>[2x]AFLHVGAQLGTELFIVRQLLQIVKQKTNQNSVDTTLKFTLSALWNLTDESPTTCRHFIENQGLELFMRVLESFPTESS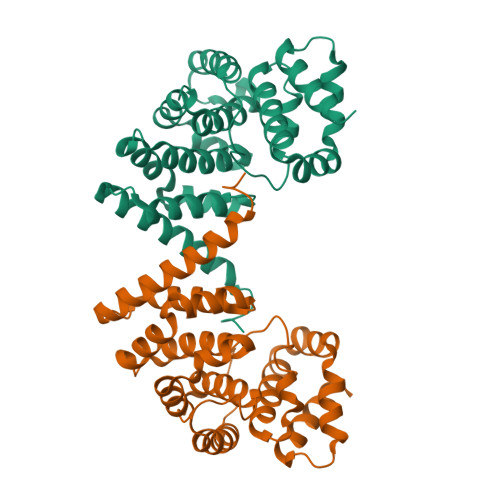IQQKVLGLLNNIAEVQELHSELMWKDFIDHISSLLHSVEVEVSYFAAGIIAHLISRGEQAWTLSRSQRNSLLDDLHSAILKWPTPECEMVAYRSFNPFFPLLGCFTTPGVQLWAVWAMQHVCSKNPSRYCSMLIEEGGLQHLYNIKDHEHTDPHVQQIAVAILDSLEKHIVR>[3x]GGCGAAGAACCGGGGAGCC

One especially common junction element is the kink-turn (k-turn). k-turns are elements in double-stranded RNA that introduce a tight kink into the helical axis, with an included angle close to 50°. A standard k-turn comprises a three-nucleotide bulge followed by successive G•A and A•G trans G(sugar edge)•A(Hoogsteen edge) basepairs. k-turns are commonly-occurring motifs that introduce sharp kinks into duplex RNA, thereby facilitating tertiary contacts. Both the folding and conformation of k-turns are determined by their local sequence. k-turns fall into two conformational classes, called N3 and N1, that differ in the pattern of hydrogen bonding in the core. We show here that this is determined by the basepair adjacent to the critical G•A pairs.

The exceptional N1 structure is Kt-7 observed in the Haloarcula marismortui ribosomal 50S subunit. However, we have shown previously that in other environments, this k-turn (abbreviated here to HmKt-7) adopts the N3 structure. In the course of our studies of k-turns we have determined numerous structures of HmKt-7 removed from the ribosomal context including three new structures reported here, all of which are N3 structures. Moreover, the various structures, with resolutions in the range 1.7 to 3.1 Å, have been determined in five different space groups, encompassing hexagonal, tetragonal and orthorhombic symmetries. Several include multiple molecules within the asymmetric unit and altogether there are 17 independent structures, all of which are unambiguously in the N3 conformation, and all in a closely similar conformation with a small RMSD values. Thus it is clear that the N1 conformation adopted by HmKt-7 in the ribosome is the single exception. In the ribosome the k-turn mediates an important tertiary interaction, and is bound by the L24 protein, and it is likely that these factors force the conformation against its intrinsic nature.>[15x]MSNFKVRDPVIQERLDHDYAHHPLVARMNTLDQGNMSQAEYLVQKRHYLVFLIAHHYYEAYLRRMGGIQRRDHLQTLRDQKPRERADRVSAASAYDAGTFTVPSRPGPASGTTPGGQDSLGVSGSSITTL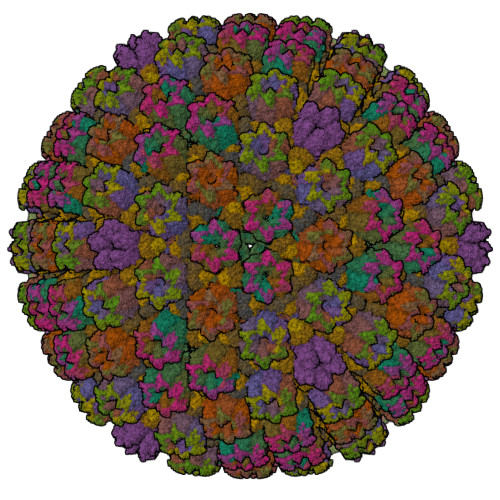SSGPHSLSPASDILTTLSSTTETAAPAVADARKPPSGKKK;>MEATLEQRPFPYLATEANLLTQIKESAADGLFKSFQLLLGKDAREGSVRFEALLGVYTNVVEFVKFLETALAAACVNTEFKDLRRMIDGKIQFKISMPTIAHGDGRRPNKQRQYIVMKACNKHHIGAEIELAAADIELLFAEKETPLDFTEYAGAIKTITSALQFGMDALERGLVDTVLAVKLRHAPPVFILKTLGDPVYSERGLKKAVKSDMVSMFKAHLIEHSFFLDKAELMTRGKQYVLTMLSDMLAAVCEDTVFKGVSTYTTASGQQVAGVLETTDSVMRRLMNLLGQVESAMSGPAAYASYVVRGANLVTAVSYGRAMRNFEQFMARIVDHPNALPSVEGDKAALADGHDEIQRTRIAASLVKIGDKFVAIESLQRMYNETQFPCPLNRRIQYTYFFPVGLHLPVPRYSTSVSVRGVESPAIQSTETWVVNKNNVPLCFGYQNALKSICHPRMHNPTQSAQALNQAFPDPDGGHGYGLRYEQTPNMNLFRTFHQYYMGKNVAFVPDVAQKALVTTEDLLHPTSHRLLRLEVHPFFDFFVHPCPGARGSYRATHRTMVGNIPQPLAPREFQESRGAQFDAVTNMTHVIDQLTIDVIQETAFDPAYPLFCYVIEAMIHGQEEKFVMNMPLIALVIQTYWVNSGKLAFVNSYHMVRFICTHMGNGSIPKEAHGHYRKILGELIALEQALLKLAGHETVGRTPITHLVSALLDPHLLPPFAYHDVFTDLMQKSSRQPIIKIGDQNYDNPQNRATFINLRGRMEDLVNNLVNIYQTRVNEDHDERHVLDVAPLDENDYNPVLEKLFYYVLMPVCSNGHMCGMGVDYQNVALTLTYNGPVFADVVNAQDDILLHLENGTLKDILQAGDIRPTVDMIRVLCTSFLTCPFVTQAARVITKRDPAQSFATHEYGKDVAQTVLVNGFGAFAVADRSREAAETMFYPVPFNKLYADPLVAATLHPLLANYVTRLPNQRNAVVFNVPSNLMAEYEEWHKSPVAAYAASCQATPGAISAMVSMHQKLSAPSFICQAKHRMHPGFAMTVVRTDEVLAEHILYCSRASTSMFVGLPSVVRREVRSDAVTFEITHEIASLHTALGYSSVIAPAHVAAITTDMGVHCQDLFMIFPGDAYQDRQLHDYIKMKAGVQTGPPGNRMDHVGYAAGVPRCENLPGLSHGQLATCEIIPTPVTSDVAYFQTPSNPRGRAACVVSCDAYSNESAERLLYDHSIPDPAYECRSTNNPWASQRGSLGDVLYNITFRQTALPGMYSPCRQFFHKEDIMRYNRGLYTLVNEYSARLAGAPATSTTDLQYVVVNGTDVFLDQPCHMLQEAYPTLAASHRVMLDEYMSNKQTHAPVHMGQYLIEEVAPMKRLLKLGNKVVY[16x];>MKVQAENAARLGRQVLGLLPPPTHRVSLTRGPEFARGVRDLLSKYAASTRPTVGSLHEALRQAPFRQPTYGDFLVYSQTFSPQEPLGTFLFSFKQEDNGSSMDMLLTPTSLFMLSGMEAAKAPQTHKVAGVWYGSGSGLADFIPNLSELMDTGEFHTLLTPVGPMVQSVHSTFVTKVTSAMKGVGLARDEPRAHVGLTLPCDMLVDLDESCPMVQRREPAGLNVTIYASLVYLRVNQRPSMALTFFQSGKGFAEVVAMIKDHFTDVIRTKYIQLRHELYINRLVFGAVCTLGTVPFDSHPVHQSLNVKGTSLPVLVFANFEAACGPWTVFL[5x];>MALDKSIVVNLTSRLFADELAALQSKIGSVLPLGDCHRLQNIQALGLGCVCSRETSPDYIQIMQYLSKCTLAVLEEVRPDSLRLTRMDPSDNLQIKNVYAPFFQWDSNTQLAVLPPLFSRKDSTIVLESNGFDIVFPMVVPQQLGHAILQQLLVYHIYSKISAGAPGDVNMAELDLYTTNVSFMGRTYRLDVDNTDPRTALRVLDDLSMYLCILSALVPRGCLRLLTALVRHDRHPLTEVFEGVVPDEVTRIDLDQLSVPDDITRMRVMFSYLQSLSSIFNLGPRLHVYAYSAETLAASCWYSPR[10x]>LPTTTVSLSAETLPDVQAGSVVLYRKFEVGEVITVRPRANAFDIDLHIKPEYRNLLTSNSVFWAEGGAKVQLNGSGLTVQASPLSRALKGAISFDNLSGASASQRKGDKRILYASETAARAVGGQITLHAFDAGKLAVGMPIRYLGIDIGQIQTLDLITARNEVQAKAVLYPEYVQTFARGGTRFSVVTPQISAAGVEHLDTILQPYINVEPGRGNPRRDFELQEATITDSRYLDGLSIIVEAPEAGSLGIGTPVLFRGLEVGTVTGMTLGTLSDRVMIAMRISKRYQHLVRNNSVFWLASGYSLDFGLTGGVVKTGTFNQFI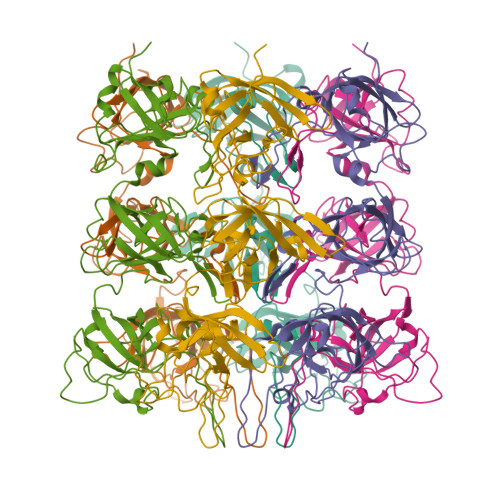RGGIAFATPPGTPLAPKAQEGKHFLLQESEPKEWREWGTALPK[6x]> MASVVAIHEAETADYILDVLVEGVKAKAGDTVEIPLKFENVPSHGIQSFNLSLYYDSKAIEVLKVEPGSIITDPANNFDYNIVYKDSEIVFLFDDDKQKGEGLIKTDGVFAKLTVRIKPDIFKDSGSTKKYSLITFGESNFCDFDLKPILAVLKEGKVEIE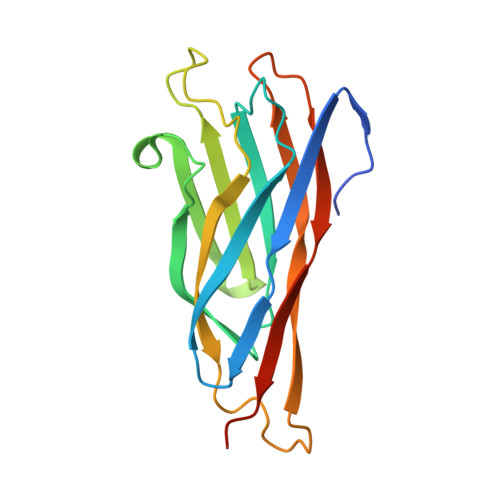KLEHHHHHH>[5x]MFPTGWRPKLSESIAASRMLWQPMAAVAVVQIGLLWFSPPVWGQDMVSPPPPIADEPLTVNTGIYLIECYSLDDKAETFKVNAFLSLSWKDRRLAFDPVRSGVRVKTYEPEAIWIPEIRFVNVENARDADVVDISVSPDGTVQYLERFSARVLSPLDFRR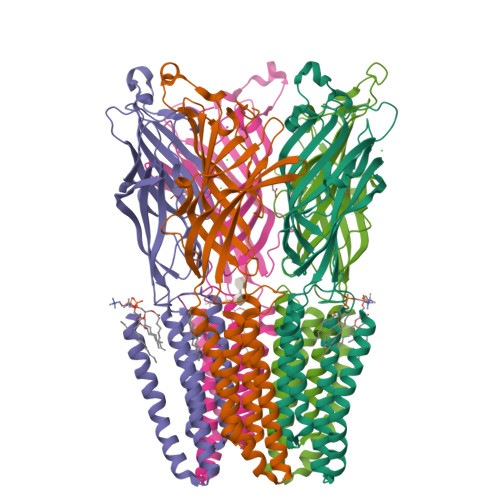YPFDSQTLHIYLIVRSVDTRNIVLAVDLEKVGKNDDVFLTGWDIESFTAVVKPANFALEDRLESKLDYQLRISRQYFSYIPNIILPMLFILFISWTAFWSTSYEANVTLVVSTLIAHIAFNILVETNLPKTPYMTYTGAIIFMIYLFYFVAVIEVTVQHYLKVESQPARAASITRASRIAFPVVFLLANIILAFLFFGF> MGASDDLTIEILTDDADYDLQRFDCGEEALNLFLTTHLVRQHRNKILRAYILCRNTPERQVLGYYTLCGSCFERAALPSK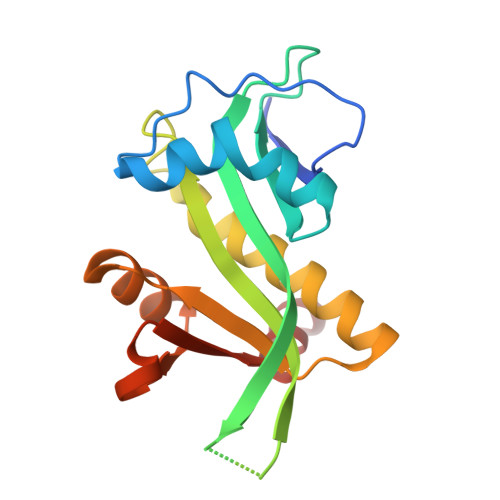SKQKKIPYKNIPSVTLGRLAIDRSLQGQGWGATLVAHAMNVVWSASLAVGIHGLFVEALNEKAHTFFKSLGFIPLVGENENALFFPTKSIELLFTQSD>[10x]ANATKTVPQLSTITPRFLLHLLSWVPVEAGIYRVNRVVNPDRVAIHSEAGAGTEEPLPETYVDYETHPREYTLRSISTLLDVHTRVSDLYSSPHDQVTQQLRLTIETIKERQEYELVNNPEYGLLAQATPEQTIQTLAGAPTPDDLDALITKVWKTPAFFLTHPLGVAAFGRECTYRGVPPPTVSMYGAQFITWRGIPIVPSDKVPVEDGTTKFVLVRTGEERQGVVGLFQPGLVGEQAPGLS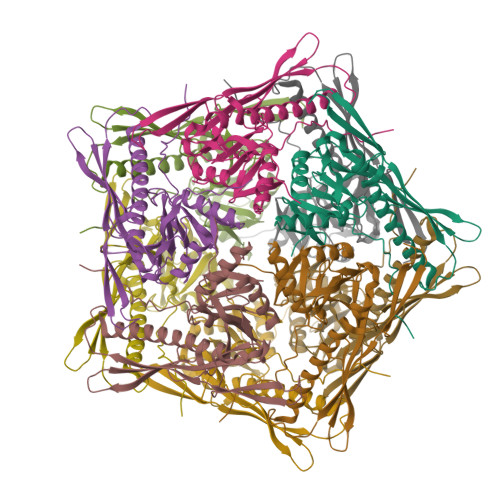VRFTGINRSAIASYLVTLYTSLAVLTDDALAVLDGVAVDQFHEYQ>MKKKDTCEIFGYDEEKVNRIQGDLQTVDISGVSQILKAIADENRAKITYALCQDEELCVCDIANILGVTIANASHHLRTLYKQGVVNFRKEGKLALYSLGGEAIRQIM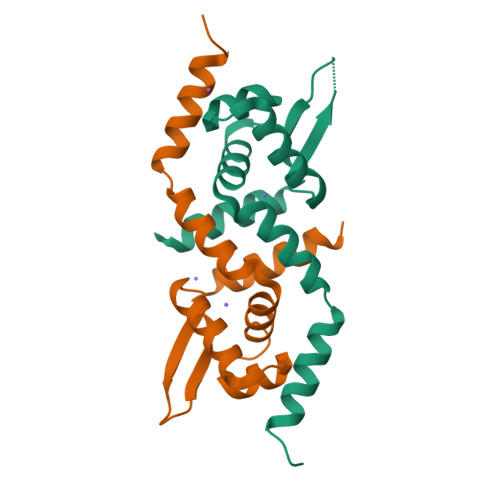MIALAHKKEVKVNV[6x]5-(4-oxo-2-phenyl-1,5,7,8-tetrahydropyrido[4,3-d]pyrimidine-6(4H)-carbonyl)-1,3-dihydro-2H-2lambda~6~,1-benzothiazole-2,2-dione 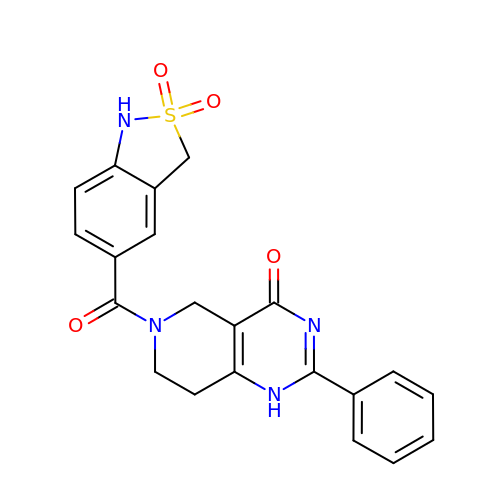| C21 H18 N4 O4 S | XRENRYGQQDHQAY-UHFFFAOYSA-N> Q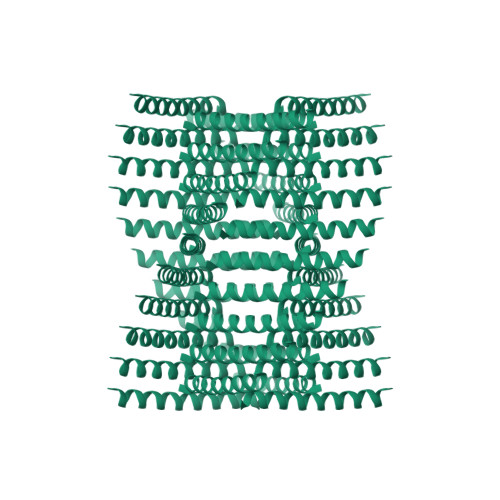AEILKADAENNRAYARILEAHAEILKAQ2-[[(2~{S})-2-decanoyloxypropoxy]-oxidanyl-phosphoryl]oxyethyl-trimethyl-azanium 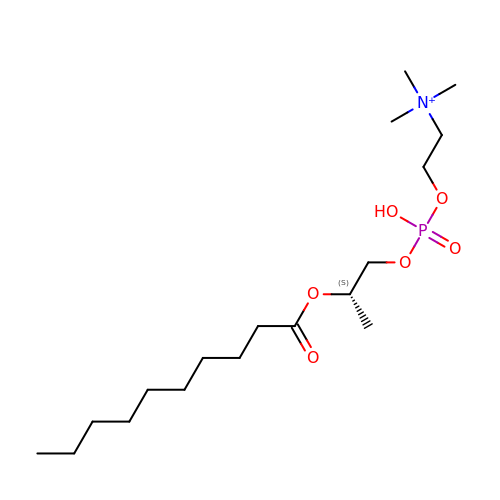| C18 H39 N O6 P | QDKXDMCUNRVOEC-KRWDZBQOSA-O>GAEIYNKD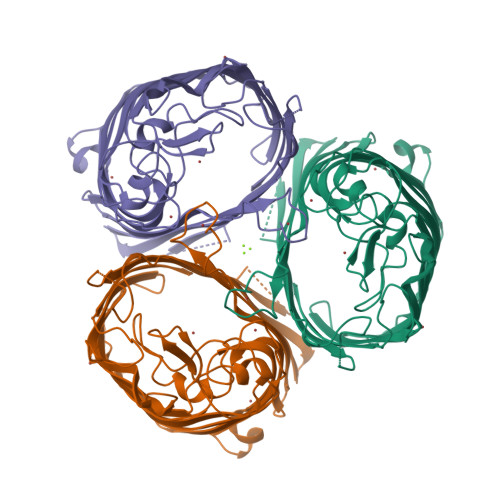GNKVDLYGKAVGLHYFSKGNGENSYGGNGDMTYARLGFKGETQINSDLTGYGQWEYNFQGNNSEGADAQTGNKTRLAFAGLKYADVGSFDYGRNYGVVYDALGYTDMLPEFGGDTAYSDDFFVGRVGGVATYRNSNFFGLVDGLNFAVQYLGKNERDTARRSNGDGVGGSISYEYEGFGIVGAYGAADRTNLQEAQPLGNGKKAEQWATGLKYDANNIYLAANYGETRNATPITNKFTNTSGFANKTQDVLLVAQYQFDFGLRPSIAYTKSKAKDVEGIGDVDLVNYFEVGATYYFNKNMSTYVDYIINQIDSDNKLGVGSDDTVAVGIVYQF[2x]>MERFLLNSTVLLYRLSTVSLDEVSLDERVESSVFLAQYEQARSLPDHVAKSAWSYLVQQIKQRNMKLGPVAILRLIAEKFIKNEKGGPKIDLPMFSEWQTLMSRVSCLPIIACHQVFNPGPASQEYSFRWPLYPYHPTVEDYITRECLHETHQHLNGSTSAEECWLDALKHPEACLRDFEKGWASQEMKQLCAQIDPSLTPRIFKDRLQIACNIREILCRVAQGVELPEWIASMQNPQQLANSTILHNGREYGFATVWPIDDKYSQESEFCWLTGLLEKWRFNAPEGLERLLWIYLLIQNQYLTLLVQRDDFFGFEQFQNYTMTELREETEKSYLSRFKHAHGAGVYSQVRYLEGRFAPKSDPNKMQKLLFSVLRGYWEYLSAHMSMEWVHEKPLTISQVLDNLELVEPHGKCVELALVPHFIKRKPKNGEAYPHALLFKDLKNQAAILMDMLKSEPRLTGWIRGVDAAANEMHAPPELFCPLFRVLAKSGIAHFTYHVGEDFPHLISGIRSIDDALRFLPLRNGDRLGHCTAIGITPSIWKRSLPLSLSMTKETRLLDLVFIWRELRSHPELLRYASDAAIEAVRLAHKVFSLEEEVSITTLDQVFEMRGLLAESEGLLSELNEPLKPKSLWLEEYERARELVKTTGMKRPLKLYKQWLTSDNVRKQRAEYVEVALEYLPDEAVVALQQAVMAKMADRNIAIECPPTSNTRISQYRNVSEHHIFRWMGLPGEAIEGDVPMSICLGSDDPGIFAADLKSEFYHLFVVLTRKFGLSPADALRKVAEVNENGRIYRFHDVS[12x];>[7x]MTDSVQTETTKGKIIINLFAPNLSGSTKEDDLIQKSLRDQLVESIRNSIAYPDTDKFAGLTRFIDEPGRNVFFVDGTRGAGKTTFINSVVKSLNSDQDDVKVNIKCLPTIDPTKLPRHEPILVTVTARLNKMVSDKLKGYWASNDYRKQKEQWQNHLAQLQRGLHLLTDKEYKPEYFSDALKLDAQLDYSIGGQDLSEIFEELVKRACEILDCKAILITFDDIDTQFD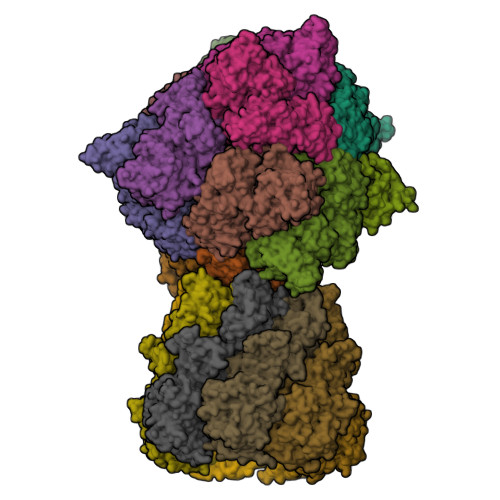AGWDVLESIRKFFNSRKLVVVATGDLRLYSQLIRGKQYENYSKTLLEQEKESVRLAERGYMVEHLEQQYLLKLFPVQKRIQLKTMLQLVGEKGKAGKEEIKVKTEPSMQDIDAIDVRQAIGDAVREGLNLREGSDADMYVNELLKQPVRLLMQVLQDFYTKKYHATSVKLDGKQSRNERPDELSVPNLLRNALYGSMLSNIYRAGLNYEQHRFGMDSLCKDIFTYVKQDRDFNTGFYLRPQSESEALRNCSIYLASQVSENCQGSLSKFLQMLLVGCGSVSIFNQFVTELARAENDREKFEQLISEYVAYMSVGRIESASHWANRCCAVVANSPNDEKIGVFLGMVQLNRKSRQNMPEGYKKFNIDTENGLAKAAMASSLSTVASNNLMDFCSVFNLIGAIADISACRCERSAITNAFNKVIAQTTCIVPPWSEAAVRAEMKGSSKSADNDAAVLDVDLDPKDDGVIDESQQDDATEFSDAITKVEQWLKNVNEIEIGIRPSALLIGKVWSRFYFNLNNVADQHKTRLYRNAEHGRMASQSNAAKIMRFNVLAFLHAVLVEESLYHSVSDREYIGEGLRLNPVTSVDEFEKKIKIIGEKLKADNKTWKNTHPLFFLLISCPILHPFIFPIGGINCSVKALNKETSFNKLIDEIVGDKLLSDEEWDYLTKNNDQKTNTRQQIFQNTITSLNSSTIVGASYDKDTPARKTKSPSLGDSEEK Globulins belong to cupin superfamily and are categorized as 11–12S legumin and 7–8S vicilin based on its sedimentation coefficients. Vicilins are trimeric protein expressed by multiple structural genes and their extensive post-translational processing (glycosylation and protease action) results in a high degree of polymorphism. In this study, we have structurally and functionally characterized a 52 kDa protein from the seeds of Mc. The crystal structure of Momordica charantia 7S (Mc7S) globulin showed maximum homology to 7S vicilins.

The crystal structure of protein was determined at a final resolution of 3.1 Å. It belongs to P63 space group and has a single monomer in an asymmetric unit. The monomer of Mc7S comprises of two cupin fold polypeptide chain separated by a pseudo-dyad axis of symmetry as observed in the other 7S family members. The trimer was observed when the three monomer molecules were arranged in the form of an equilateral triangle where their extended α-helix regions interact with the other monomer in a head-to-tail fashion. Four stretches (I: 125–127 residues, II: 215–220 residues, III: 225–247 residues, and IV: 325–334 residues) were omitted from the final model because no electron density at the main-chain level was available. The structural analysis led to the identification of a bound copper and acetate ion in the protein. The Fo-Fc map showed the clear electron density near the tyrosine (Tyr49) from the N-terminal domain and the cysteine (Cys321), and two histidines (His323 and His355) from the C-terminal domain. The copper ion is placed slightly away from the centre of the trigonal plane formed by SG of Cys321, ND1 of His323, and the NE2 of His374. The metal possesses a trigonal planar geometry with copper in the centre as inferred from CheckMyMetal server. The acetate interacts with NE2 atom of His299 and ND2 atom of Asn301 through its O atom.

> HNPYYFHEHSFQSRFRSEDGHWRVLERFSQRSDVLRGIENNRFAILEARPQTFIIPHHLDAETVLLVVRGRAAITTVVQERKETKRESYNAERGDVMVIPAGATIYLVNHENEDLQIVKLIQPINNPGEFKDYLSAGGEDQSYYTVFSNDVLEAALDIPRDRLERVFKQHSERRGKIIKGSQEQLKALSQRATSVRKGGRGTRALIKLENQTPVYSNQYGQMFEACPDEFPQLQRTNVAAAIVDIKQGGMMVPHFNSRATWAVFVAEGAGSFEMACPHLEESEGRSSRFERVAGHLSPGGLLVVPAGHPIAVMASPKENLRLVGFGINAQNNLRNFLAGKENIMNEVDQEAKELTFNIKGKEADEIFKSQRESFFTKGPVG>[4x]MSLKI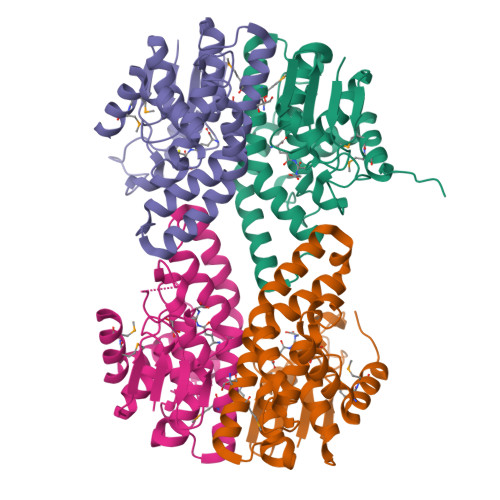YGVYRSRASRPLWLLAELDLPFEHVPVIQANRVAHPHGPEAPLNTASAAYLAVNPLGQIPCLEEEGLILTESLAITLHIARTQGGQLGPRSEPEDALMVSWSLFAATAVEPPALEIQLIQRSGGGTSPEGQAAIAIAAERLRRPLARLERHFAAEDYLVGGRFTVADLNLAETLRYGQAHPALLEPFPAVAAWLDRCQSRPAFRLMMERRAAEGHHHHHH>SFTMSGGFELQPRDGGPRVALAPGETVIGRGPLLGITDKRVSRRHAILEVAGGQLRIKPIHTNPCFYQSSEKSQLLPLKPNLWCYLNPGDSFSL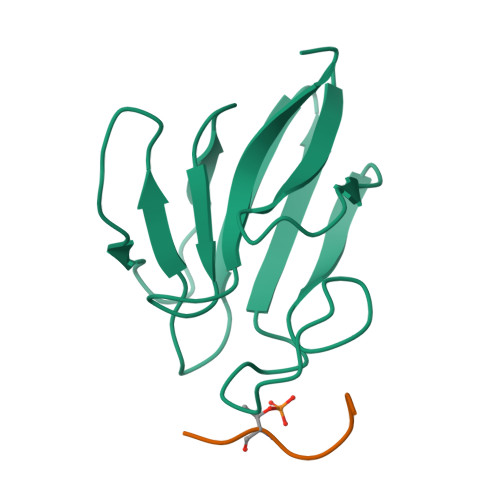LVDKYIFRILSIPS[2x];>[2x]PYAGETDE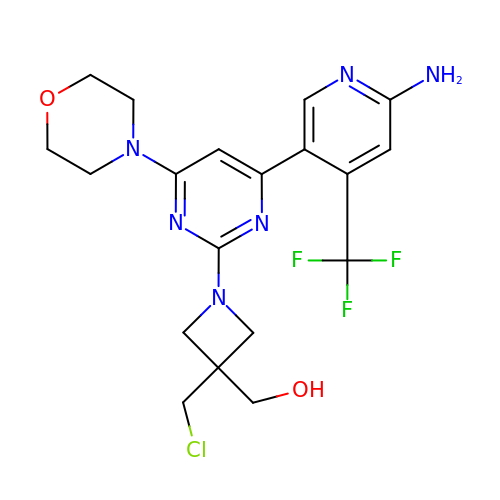[1-{4-[6-amino-4-(trifluoromethyl)pyridin-3-yl]-6-(morpholin-4-yl)pyrimidin-2-yl}-3-(chloromethyl)azetidin-3-yl]methanol | C19 H22 Cl F3 N6 O2 | JQPAIKDXQCXSKJ-UHFFFAOYSA-N As a scaffold for aromatic cluster design, we chose ferritin as a protein cage platform with a 12 nm outer diameter and an 8 nm inner cavity, composed of 24 subunits. To prove this concept through protein engineering, we focused on a two‐fold symmetric inter‐subunit interface of a recombinant horse spleen apo‐L ferritin (Fr) as a target region for mutagenesis. Herein, we present the construction of an aromatic cluster with an artificial molecular binding pocket at the two‐fold symmetric interface of ferritin and explore its ligand‐binding characteristics. We developed a system that uses ligand binding as a driving force to induce and propagate changes in the orientation of multiple aromatic side chains.

The resulting mutants were named Fr‐F2 (Fr‐E56F/R59F), Fr‐F4 (Fr‐R52F/E56F/R59F/E63F), and Fr‐F6 (Fr‐E53F/E56F/E57F/R59F/E60F/E63F), where i in Fr‐Fi represents the number of newly introduced Phe residues per ferritin monomer (upper). The largest number was obtained for NR•Fr‐F6, showing 10.4 molecules of NR are encapsulated per protein cage. This amount is in good agreement with the number of the pockets at the two‐fold symmetric interface in the ferritin cage, suggesting that 12 pockets of Fr‐F6 are occupied by approximately one molecule of NR. Analysis of the 2Fo‐Fc maps revealed electron densities corresponding to Nile Red (NR) at the two‐fold symmetric interfaces of NR•Fr‐F1, NR•Fr‐F2, NR•Fr‐F4, and NR•Fr‐F6, observed as overlapping densities due to the interface symmetry. NR was positioned between two F59 residues, forming π–π stacking interactions in an F59–NR–F59' configuration. Anion‐π interactions between NR and E60 in NR•Fr‐F1 and NR•Fr‐F2, and CH‐π interactions between NR and F60 in NR•Fr‐F6, were identified, indicating NR's stabilization in the F59–F59' pocket via multiple non‐covalent interactions. Upon comparing the protein structures before and after Nile Red (NR) encapsulation, orientational changes of Phe side chains were observed in NR•Fr‐F6 due to NR binding. In NR•Fr‐F6, compared to Fr‐F6 without NR, the occupancy of the alternate conformation of F60 and F56 changed from 0.3 to 0.7 and 0.3 to 0.5, respectively. The dihedral angles χ1 (defined by the N–Cα–Cβ–Cγ torsion) of the F56 and F60 side chains, which directly interact with NR, changed by 219° and 102°, respectively. Since the residue F57 and F53 have tendency to form double conformation having weak density of the alternate confer, this might be an indication that the rotational movements of F56 and F60 upon NR binding propagate to F57 and F53.

> SSQIRQNYSTEVEAAVNRLVNLYLRASYTYLSLGFYFDRDDVALEGVCHFFRFLAFFKFFGAFRLLKMQNQRGGRALFQDLQKPSQDEWGTTLDAMKAAIVLEKSLNQALLDLHALGSAQADPHLCDFLESHFLDEEVKLIKKMGDHLTNIQRLVGSQAGLGEYLFERLTLKHD(6alpha,8alpha)-6-(pent-2-yn-1-yloxy)androsta-1,4-diene-3,17-dione | C24 H30 O3 | 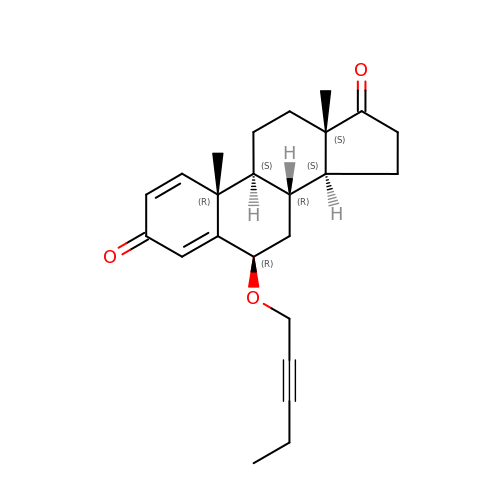VZGAHAQWKVTWEF-RAPVPNNWSA-N> MEALAKEIGIPEGEYREIVQRLGREPNRVELLLFKVMWSEHCAYKNSRPLLKALPKEGEAVLQGPGENAGVVRVGEGWAVAFKIESHNHPSAVEPFQGAATGVGGILRDIMSMGARPIALLDSLRFGPPEEARSRYLLKGVVSGIAFYGNAIGVPTVGGDLYFHEGYRENPLVNAMCLGLLREEHLKRSRASLGRPIYYAGAKTGRDGI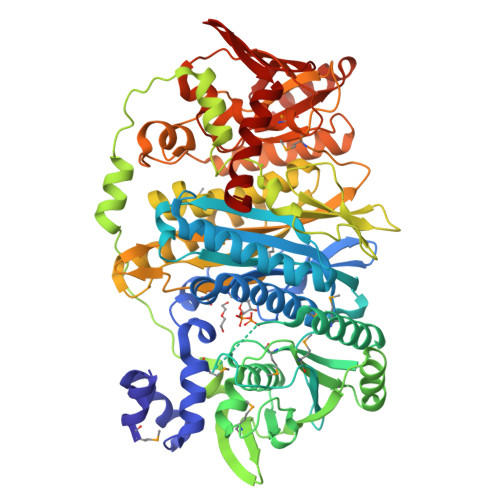GGAAFASRELKEEKAEDRPAVQVGDPFLGKLLMEATLEAIELDLVEGVQDMGAAGLTSSLSELAHKSGLGVELHLDLVPTREEGMTPEELLLSESQERMVLVPKEGKEKALEEVFGRWGLDCVPVARTIPERVFRVLFRGEVVAEVPTEALAEAPTYVRVGREDPEVRRLRETPIPPLEADPQEVLRRLLASPNLASREAVYERYDHQVGTRTALLPGKGDAAVLWIKGTRLGVAAKVDQNPRYSRLHPRLGAMHALAEACRNVSVVGAKPLAYTDGLNLGSPETPEGYHELAETIAGLKEASEALGVPVVSGNVSLYNESGGKRIPPTAMVGVVGVLEVDKRAEMGFRRPGEVLLLIGEERGELGASEVLYLLTGKEFGHPPRLDLGREKAVQEAIRDLIQRGLTRTAHDVAEGGLLLALAEMTFPYGVGATVEVREEGLEALFGEAPSRVLFTVEKTRLQEATLLLEERGLPYRVLGETGGKSLTVLTPGGVLEWSLEELLSAWKAPLREVLDG>[2x]KDITDKNQSIDSGISSLSYNRNEVLASNGDKIESFVPKEGKKAGNKFIVVERQKRSLTTSPVDISIID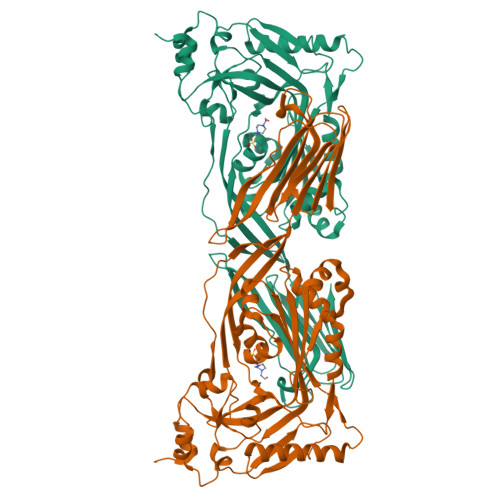SVNDRTYPGALQLADKAFVENRPTILMVKRKPININIDLPGLKGENSIKVDDPTYGKVSGAIDELVSKWNEKYSSTHTLPARTQYSESMVYSKSQISSALWVNAKVLENSLGVDFNAVANNEKKVMILAYKQIFYTVSADLPKNPSDLFDDSVTFNDLKQKGVSNEAPPLMVSNVAYGRTIYVKLETTSSSKDVQAAFKALIKNTDIKNSQQYKDIYENSSFTAVVLGGDAQEHNKVVTKDFDEIRKVIKDNATFSTKNPAYPISYTSVFLKDNSVAAVHNKTDYIETTSTEYSKGKINLDHSGAYVAQFEVAWDEVSYDKEGNEVLTHKTWDGNYQDKTAHYSTVIPLEANARNIRIKAREATGLAWEWWRDVISEYDVPLTNNINVSIWGTTLYPGSSITYN(6-methoxy-1-benzofuran-3-yl)acetic acid | C11 H10 O4 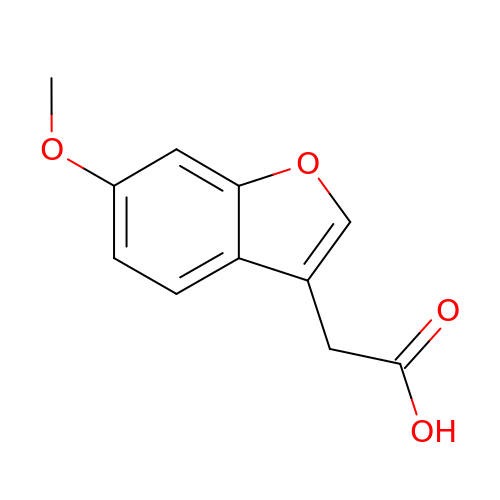| QCXJFLREQGIACT-UHFFFAOYSA-N3-[5-chloranyl-2-oxidanylidene-6-[(1~{R})-1-pyridin-2-ylethoxy]-1,3-benzoxazol-3-yl]propanoic acid | C17 H15 Cl N2 O5 | 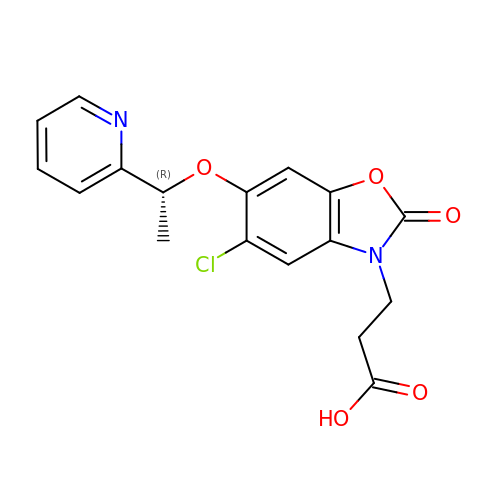PVGOQRJICUIPTG-SNVBAGLBSA-N In the barley β-d-glucan glucohydrolase, a glycoside hydrolase family 3 (GH3) enzyme, the Trp286/Trp434 clamp ensures β-d-glucosides binding, which is fundamental for substrate hydrolysis during plant growth and development. HvExoI folds into a two-domain structure consisting of an (α/β)8 barrel (domain 1) and an (α/β)6 sandwich (domain 2) with a 13 Å-deep active site pocket embracing the subsites −1 and +1, positioned at the interface between the two domains. HvExoI catalyses the hydrolytic removal of nonreducing glucose (Glc) moiety from a broad spectrum of poly- and oligomeric β-d-glucosides. The crucial role of substrate binding in HvExoI implies a pair of the aromatic Trp286 and Trp434 residues that form a clamp at the +1 subsite, which is positioned next to a pocket-shaped site at the −1 subsite, housing the Asp285 and Glu491 catalysts.

G4SG-OMe bound to native and WT recombinant HvExoI with the Ki values of 1.0 ×10−3 M. The β-d-glucopyranose rings of thio-saccharide analogues at the −1 subsites in the WT crystal structure complexes were engaged in H-bond networks and observed in the 4C1 conformation for G2SG-OMe and G6SG-OMe, the 4H3 conformation for 4NP-G3SG, and the 4E/4H3 conformations for G4SG4OG, while the β-d-glucopyranose moieties of thio-ligands at the +1 subsites adopted the 4C1 conformation. In these WT complexes, the Glc moiety at the −1 subsite was oriented almost identically, contrary to the Glc moiety at the +1 subsite that adopted various orientations. The complex with G4OG3OG was generated based on the WT HvExoI:G4SG4OG complex, upon replacing G4 with G3.

> HHAADYVLYKDATKPVEDRVADLLGRMTLAEKIGQMTQIERLVATPDVLRDNFIGSLLSGGGSVPRKGATAKEWQDMVDGFQKACMSTRLGIPMIYGIDAVHGQNNVYGATIFPHNVGLGATRDPYLVKRIGEATALEVRATGIQYAFAPCIAVCRDPRWGRCYESYSEDRRIVQSMTELIPGLQGDVPKDFTSGMPFVAGKNKVAACAKHFVGDGGTVDGINENNTIINREGLMNIHMPAYKNAMDKGVSTVMISYSSWNGVKMHANQDLVTGYLKDTLKFKGFVISDWEGIDRITTPAGSDYSYSVKASILAGLDMIMVPNKYQQFISILTGHVNGGVIPMSRIDDAVTRILRVKFTMGLFENPYADPAMAEQLGKQEHRDLAREAARKSLVLLKNGKTSTDAPLLPLPKKAPKILVAGSHADNLGYQCGGWTIEWQGDTGRTTVGTTILEAVKAAVDPSTVVVFAENPDAEFVKSGGFSYAIVAVGEHPYTETKGDNLNLTIPEPGLSTVQAVCGGVRCATVLISGRPVVVQPLLAASDALVAAWLPGSEGQGVTDALFGDFGFTGRLPRTWFKSVDQLPMNVGDAHYDPLFRLGYGLTTNATKKY>MKLIWSEESWDDYLYWQETDKRIVKKINELIKDTRRTPFEGKGKPEPLKHNLSGFWSRRITEEHRLVYAVTDDSLLIAACRYHY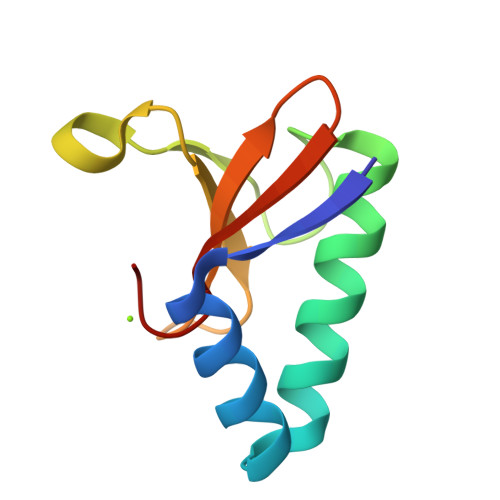[6x]>MEHRAFKWPQPLAGNKPRIWYGGDYNPDQWPEEVWDEDVALMQQAGVNLVSVAIFSWAKLEPEEGVYDFDWLDRVIDKLGKAGIAVDLASGTASPPMWMTQAHPEILWVDYRGDVCQPGARQHWRATSPVFLDYALNLCRKMAEHYKDNPYVVSWHVSNEYGCHNRFDYSEDAERAFQKWCEKKYGTIDAVNDAWGTAFWAQRMNNFSEIIPPRFIGDGNFMNPGKLLDWKRFSSDALLDFYKAERDALLEIAPKPQTTNFMVSAGCTVLDYDKWGHDVDFVSNDHYFSPGEAHFDEMAYAACLTDGIARKNPWFLMSHSTSAVNWRPTNYRLEPGELVRDSLAHLAMGADAICYFQWRQSKAGAEKWHSAMVPHAGPDSQIFRDVCELGADLNKLADEGLLSTKLVKSKVAIVFDYESQWATEHTATPTQEVRHWTEPLDWFRALADNGLTADVVPVRGPWDEYEAVVLPSLAILSEQTTRRVREYVANGGKLFVTYYTGLVDDRDHVWLGGYPGSIRDVVGVRVEEFAPMGTDAPGTMDHLDLDNGTVAHDFADVITSVADTAHVVASFKADKWTGFDGAPAITVNDFGDGKAAYVGARLGREGLAKSLPALLEELGIETSAEDDRGEVLRVERADETGENHFVFLFNRTHDVAVVDVEGEPLVASL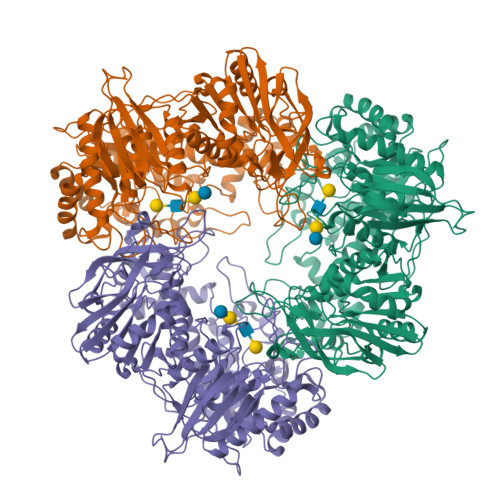AQVNESEHTAAIQPNGVLVVKLAAALEHHHHHH[2x]> GFKFVLEHDSEYQPEVKVTSYKNAIGTETDGFDSGPVFGGGTIYNVPVSLSYDRQKVYVEMPKSYTLAGDIILIDDGTLLVIKETQVLCFKMSDAK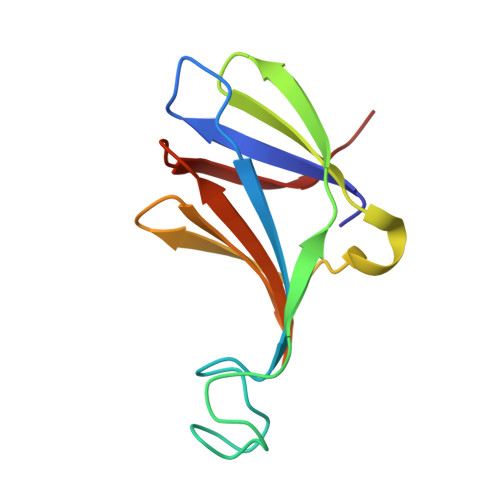ITKGYVFVA>MKKLLNTLYVTQPDTYLSLDGDNVVLLKEQEKLGRLPLHNLEAIVGFGYTGASPALMGYCAERNISITFLTKNGRFLARVVGESRGNVVLRKTQYRISENDQESTKIARNFITGKVYNSKWMLERMTREHPLRVNVEQFKATSQLLSVMMQEIRNCDSLESLRGWEGQAAINYNKVFDQMILQQKEEFAFHGRSRRPPKDNVNAMLSFAYTLLANDVAAALETVGLDAYVGFMHQDRPGRASLALDLMEELRGLYADRFVLSLINRKEMTADGFYKKENGAVLMTDEARKTFLKAWQTKKQEKITHPYLGEKMSWGLVPYVQALLLARFLRGDLDEYPPFLWK[4x];>GSMLVLITYDVQTSSMGGTKRLRKVAKACQNYGQRVQNSVFECIVDSTQLTSLKLELTSLIDEEKDSLRIYRLGNNYKTKVEHIGAKPSIDLEDPLIF[2x];>ASNEEDRYLMLSGLQHFQFCKRQWALIHIEQQWEENVRTIEGQHLHKKADQPFMKEKRGSKLTVRAMPIQSKNLQISGICDVVEFVQDSEGIELSGVSGSYKAFPVEYKRGKPKKGDEDIVQLVAQAMCLEEMLVCRIDKGYLFYNEIKHRVEVPITDALRDKVVQMAKEMHHYYENRHTPKVKTGPFC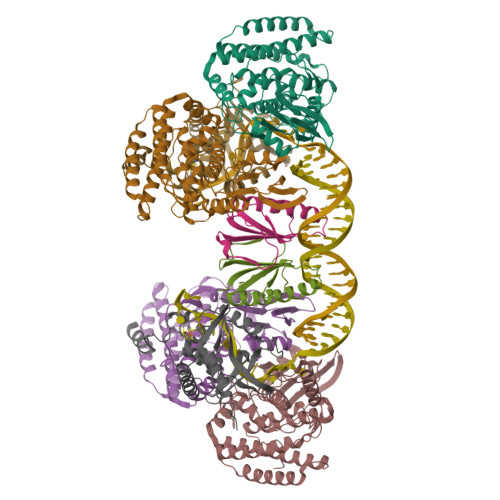NNCSLQSICLPKLMNKRSVKRYIEGRLSE[2x]>[2x]MSAFFLNMEKSIITQKIIAKAFKDLMQSNAYHQISVSDIMQTAKIRRQTFYNYFQNQEELLSWIFENDFAELINDNSDYYGWQNELLLLLRYLDENQIFYQKIFVIDKNFEHFF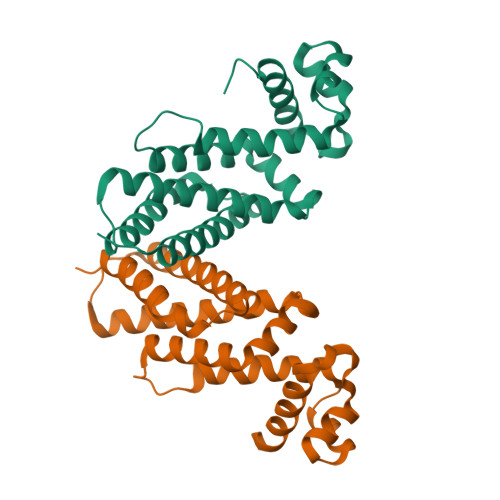LIQWENLLDKVIFDQEKKSDYHWSDLEKSFICRYNAAAICAITRESIIRGNSLEKLYSQIVNLLLAQIKIFESLEHHHHHH> PWSEFRLTPAEAAAAAALAARCAQRYDE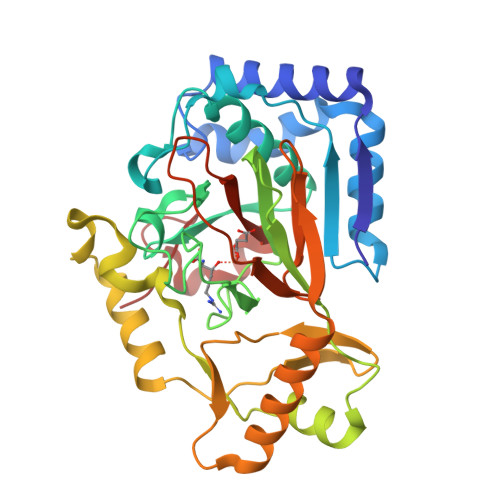TDGPEFLLDAPVIAHELPRRLRTFMARARLDAWPHALVVRGNPVDDAALGSTPVHWRTARTPGSRPLSFLLMLYAGLLGDVFGWATQQDGRVVTDVLPIKGGEHTLVSSSSRQELGWHTEDAFSPYRADYVGLLSLRNPDGVATTLAGVPLDDLDERTLDVLFQERFLIRPDDSHLQVNNSTAQQGRVEFEGIAQAADRPEPVAILTGHRAAPHLRVDGDFSAPAEGDEEAAAALGTLRKLIDASLYELVLDQGDVAFIDNRRAVHGRRAFQPRYDGRDRWLKRINITRDLHRSRKAWAGDSRVLGQR3',6'-DIHYDROXY-3-OXO-3H-SPIRO[2-BENZOFURAN-1,9'-XANTHENE]-6-CARBOXYLIC ACID | C21 H12 O7 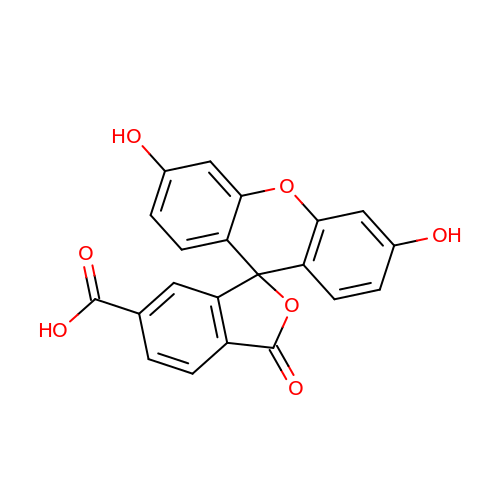| BZTDTCNHAFUJOG-UHFFFAOYSA-N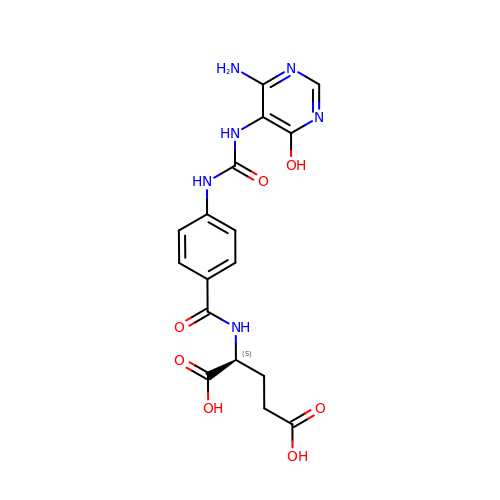(2S)-2-[[4-[(4-azanyl-6-oxidanyl-pyrimidin-5-yl)carbamoylamino]phenyl]carbonylamino]pentanedioic acid | C17 H18 N6 O7 | OUMOQELZARCDHX-JTQLQIEISA-N> MSTEAHPTVQGCLVSFPTPHILLLTLNRPEKRNCISLATSAEIQRLWTWFDTQPALYVAIITGTGESFCAGADLKEWNDLNARGITNEMTAPGLAGLPRRRGSKPIIAAVNGYCLGGGFEMVANCDIVVASENATFGLPEVQRGIAAVAGSLPRLVRVLGKQRAAEIALSGLSFSASQLER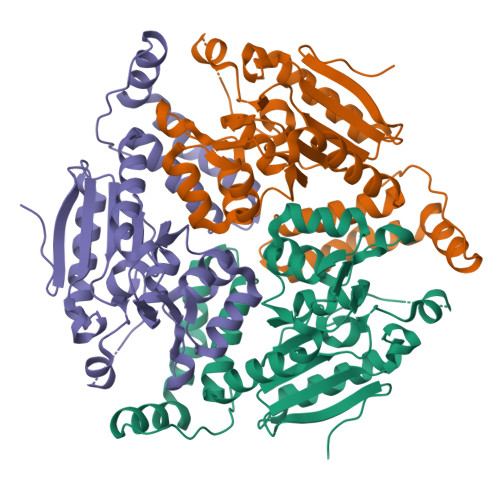WGLVNRVVEHDQLLATAVEIATAISRNSPDSVRVTMEGLHYGWEMASVEEASSALVDQWYAKLMAGENFHEGVRAFVEKRKPQWRPSKL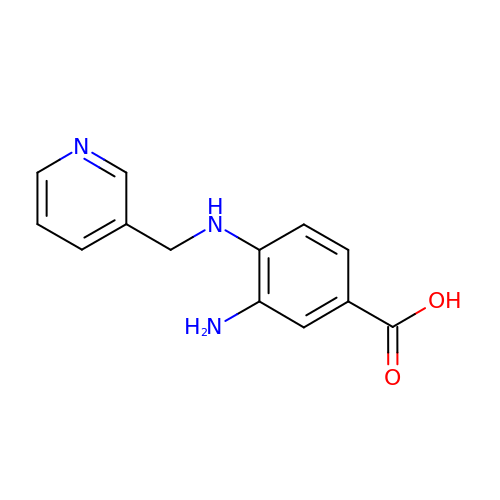3-azanyl-4-(pyridin-3-ylmethylamino)benzoic acid | C13 H13 N3 O2 | MHWWFBSFFVDUPF-UHFFFAOYSA-N1-methyl-3-oxidanyl-pyridin-2-one 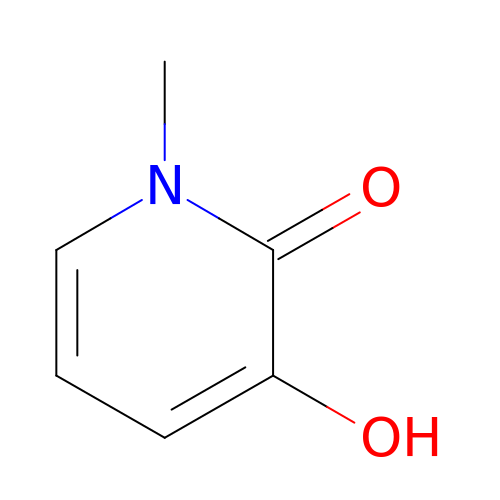| C6 H7 N O2 | QUKDWRYJPHUXQR-UHFFFAOYSA-N Interleukin (IL-), an IL-6 family cytokine, has pivotal roles in autoimmune diseases, fibrotic complications, and solid cancers. IL-11 activates downstream signalling pathways by binding its two cell surface receptors: the IL-11 specific receptor, IL-11Rα, and the signal-transducing receptor, glycoprotein (gp)13013,26. Following the formation of the receptor complex, the Janus kinase (JAK)/signal transducer and activator of stat (STAT) and extracellular signal regulated kinase (ERK)/mitogen-activated protein kinase (MAPK) pathways are primarily activated. IL-11 and IL-6 utilise a homodimer of gp13026,34,35 while other IL-6 family members exploit a heterodimer of gp130 with a second signal-transducing receptor, such as LIF receptor (LIFR), OSM receptor (OSMR), IL-27R/WSX-1 or IL-12 receptor β−2 subunit (IL-12Rβ2).

To understand the molecular mechanisms underpinning human IL-11 signalling complex formation, we solved three structures of the complex containing either the cytokine binding domains of gp130 (gp130D1-D3) or the complete extracellular domains of gp130 (gp130EC) using electron cryo-microscopy (cryo-EM) and X-ray crystallography. We obtained a 3.5 Å resolution cryo-EM reconstruction of the IL-11Δ10/IL-11RαD1-D3/gp130D1-D3 complex (referred to as the gp130D1-D3 complex), and a 3.8 Å resolution cryo-EM reconstruction of the IL-11Δ10/IL-11RαD1-D3/gp130EC complex (referred to as the gp130EC complex). D1 of IL-11Rα was not visible in the gp130D1-D3 complex map and was poorly defined in the gp130EC complex map, suggesting this domain is flexible. N-linked glycans were visible on IL-11Rα (N105, N172) and gp130 (N21, N61, N135) in all structures. Our structures of the IL-11 signalling complex allow precise identification of the interactions forming the complex. Overall, complex formation results in the burying of ~6450 Å2 of surface area. Initial formation of a 1:1 complex between IL-11 and IL-11Rα is mediated through site-I of the cytokine. The interaction between the binary IL-11/IL-11Rα complex and the first molecule of gp130 comprises two coupled interfaces: (1) between IL-11 and gp130 (site-IIA), and (2) between IL-11Rα and gp130 (site-IIB). The final interaction to form the complex is a coupled interaction between IL-11 and gp130 D1 (site-IIIA) and between IL-11Rα D2 and gp130 D1 (site-IIIB). Thus, the affinity of a single gp130 molecule at site-III is low (KD ~ mM) and it is the avidity of the symmetrically duplicated site-III interactions that maintains hexameric complex formation.

>[2x]GELLDPCGYISPESPVVQLHSNFTAVCVLKEKCMDYFHVNANYIVWKTNHFTIPKEQYTIINRTASSVTFTDIASLNIQLTCNILTFGQLEQNVYGITIISGLPPEKPKNLSCIVNEGKKMRCEWDGGRETHLETNFTLKSEWATHKFADCKAKRDTPTSCTVDYSTVYFVNIEVWVEAENALGKVTSDHINFDPVYKVKPNPPHNLSVINSEELSSILKLTWTNPSIKSVIILKYNIQYRTKDASTWSQIPPEDTASTRSSFTVQDLKPFTEYVFRIRCMKEDGKGYWSDWSEEASGITYED;>[2x]GSPDPRAELDSTVLLTRSLLADTRQLAAQLRDKFPADGDHNLDSLPTLAMSAGALGALQLPGVLTRLRADLLSYLRHVQWLRRAGGSSLKTLEPELGTLQARLDRLLRRLQLLMSRLALPQPPPDPPAPPLAPPSSAWGGIRAAHAILGGLHLTLDWAVRGLLLLKTRL;>[2x]GSSPCPQAWGPPGVQYGQPGRSVKLCCPGVTAGDPVSWFRDGEPKLLQGPDSGLGHELVLAQADSTDEGTYICQTLDGALGGTVTLQLGYPPARPVVSCQAADYENFSCTWSPSQISGLPTRYLTSYRKKTVLGADSQRRSPSTGPWPCPQDPLGAARCVVHGAEFWSQYRINVTEVNPLGASTRLLDVSLQSILRPDPPQGLRVESVPGYPRRLRASWTYPASWPSQPHFLLKFRLQYRPAQHPAWSTVEPAGLEEVITDAVAGLPHAVRVSARDFLDAGTWSTWSPEAWGTPSTGT> MAVEPFPRRPITRPHASIEVDTSGIGGSAGSSEKVFCLIGQAEGGEPNTVYELRNYSQAKRLFRSGELLDAIELAWGSNPNYTAGRILAMRIEDAKPASAEIGGLKITSKIYGNVANNIQVGLEKNTLSDSLRLRVIFQDDRFNEVYDNIGNIFTIKYKGEEANATFSV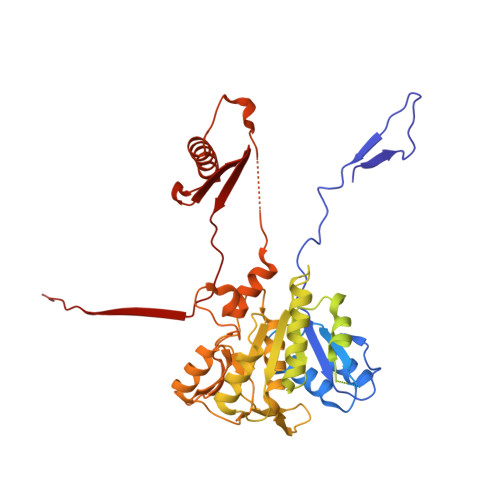EHDEETQKASRLVLKVGDQEVKSYDLTGGAYDYTNAIITDINQLPDFEAKLSPFGDKNLESSKLDKIENANIKDKAVYVKAVFGDLEKQTAYNGIVSFEQLNAEGEVPSNVEVEAGEESATVTATSPIKTIEPFELTKLKGGTNGEPPATWADKLDKFAHEGGYYIVPLSSKQSVHAEVASFVKERSDAGEPMRAIVGGGFNESKEQLFGRQASLSNPRVSLVANSGTFVMDDGRKNHVPAYMVAVALGGLASGLEIGESITFKPLRVSSLDQIYESIDLDELNENGIISIEFVRNRTNTFFRIVDDVTTFNDKSDPVKAEMAVGEANDFLVSELKVQLEDQFIGTRTINTSASIIKDFIQSYLGRKKRDNEIQDFPAEDVQVIVEGNEARISMTVYPIRSFKKISVSLVYKQQTLQA>[2x]RSENITQWNLQDNGTEGIQRAMFQRGVNRSLHGIWPEKICTGVPSHLATDTELKAIHGMMDASEKTNYTCCRLQRHEWNKHGWCNWYNIEPWILLMNKTQ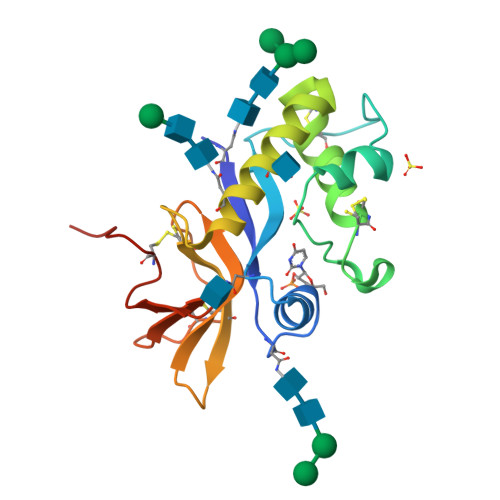ANLTEGQPLRECAVTCRYDRDSDLNVVTQARDSPTPLTGCKKGKNFSFAGILVQGPCNFEIAVSDVL> MGEDLISQEDVVVTLSHQGYVKYQPLTDYEAQRRGGKGKSAARIKEEDFIDRLLVANTHDTILCFSSRGRLYWMKVYQLPEASRGARGRPIVNLLPLEANERITAILPVREYEEGVNVFMATASGTVKKTALTEFSRPRSAGIIAVNLNDGDELIGVDLTSGSDEVMLFSAAGKVVRFKEDAVRAMGRTATGVRGIKLAGDDKVVSLIIPRGEGAILTVTQNGYGKRTAADEYPTKSRATQGVISIKVTERNGSVVGAVQVDDCDQIMMITDAGTLVRTRVSEISVVGRNTQGVILIRTAEDENVVGLQRVA

DNA Gyrase, a Type II topoisomerase, relaxes the positive helical turns by introducing negative supercoil in the DNA and prevents the overwinding of the genome. Functionally, DNA Gyrase exists as a hetero-tetramer composed of two subunits, GyraseA and GyraseB, as an A2B2 complex. GyraseA is composed of two domains, a 59kDa N-terminal domain which possesses the breakage and religation activity, and a 37kDa C-terminal domain responsible for DNA binding activity. The essential functional role of GyrA-CTD β-pinwheel fold is to wrap DNA and present G-segment for enzymatic action.

We determined the first crystal structure of GyrA-CTD from S. Typhi (StGyrA-CTD) at 2.4 Å resolution. The crystal of StGyrA-CTD (residues 530–840) diffracted upto 2.4 Å resolution and belongs to the tetragonal space group P41212 with unit cell dimensions a = b = 79.15, c = 87.36 Å. The StGyrA-CTD structure was solved by molecular replacement method using the E.coli GyrA-CTD (PDB ID 1ZI016) as a template. StGyrA-CTD adopts the β-propeller fold comprising six repeated subdomains referred to as ‘blades’ to form a β-pinwheel structure. Each blade of the pinwheel constitutes a four-stranded antiparallel β-sheet structure (A, B, C, D) linked by a 15 residue extended loop. The GyrA box region from residues 560 to 574 is an extended β2-β3 loop which could not be resolved due to poor electron density map signifying that this region is completely disordered. The electrostatic surface potential of StGyrA-CTD revealed that the positively charged residues are distributed uniformly around the perimeter of the β-pinwheel across all blades. The basic charge on the protein surface is largely contributed by the arginine and lysine residues present on the extended β2-β3 loops of all blades. This indicates that the DNA wraps around the perimeter of the StGyrA-CTD β-pinwheel structure during G-segment presentation. The sequence alignment of the individual blades depicted that the distribution and position of the charged amino acid residues in each blade in StGyrA-CTD is significantly conserved. It was observed that arginine residues, R556 (blade), R612 (blade), R667 (blade), R716 (blade), R766 (blade), and R817 (blade) could be identified as the potential DNA binding site in each blade.>GAAASGSEFMPVSVEELDATVRAFYEGRGEQQKAAQAALNQFKEDPDAWLMVDEILSRATYEQTKFLALQVLDNVIMTRWKVLPREQCQGIRNFVVQYILQCSSSEESLRTHRTLLNKLNLVLVSVLKQEWPHNWPTFINEIVSACHSSLSVCENNMIILRLLSEEVFDYSADQMTSTKTRNLKSTMCAEFSMIFQLCQEILNSATQPSLIKATLETLLRFCNWIPLGYIFETPLIDTLRTRFLEVPEFRNVTLQCLTEIGGLQTGGPGQPHTYDEQLIKMFTEVLTTISNIIPLQMDLKATYPNSNSRDQEFIQNLALFLTSFFTMHLPLIENLPNRDFLTHGHFYLIRISQIDDREIFKICLDYWLKLVQELYEEMQSLPLNDMSSMGLGMMSGGGAPNPALLEHYPLRKHKYKEVLSNLRVVMIEKMVRPEEVLIVENDEGEIVREFVKDTDSVQLYKTIRECLVYLTHLDVVDMEQIMTEKLARQVDGSEWSWHNCNVLCWAIGSISMAMNEETEKRFLVTVIKDLLGLTEMKRGKDNKAVVASNIMYIVGQYPRFLKAHWKFLKTVVNKLFEFMHESHEGVQDMACDTFIKIAKQCRRHFVALQPSENEPFIEEIIRNIGKITCDLTPQQVHTFYEACGYMVSAQGNRNQQERLLAELMAIPNAAWDEIIKAATMNPGILHEPDTIKIIGNIMKTNVSACSSIGPYFFPQIGRLYNDMLQMYAATSQLISEAVARDGEIATKMPKVRGLRTIKKEILKLVETFVEKAEDLQAVRSQMIPGLLDSVLVDYNRNVPGARDAEVLKAM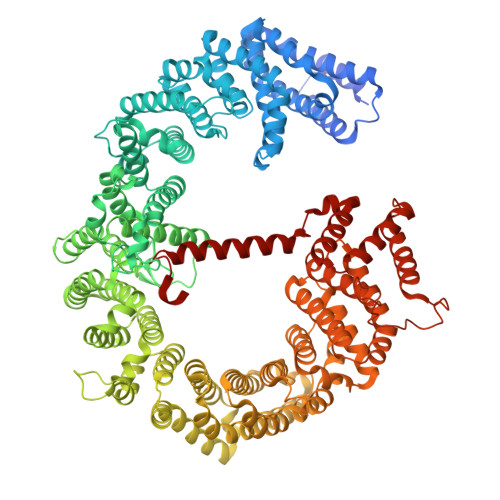TVIITRLQGLMEDQVPAIMENVFECTLDMINKDFAEYPEHRVEFFNLLRAINLYCFPALLKLDNRQFKFVIDSCMWASKHDNRDVETAGLNMCLELINNIAEKTDVQTCNAFFNQFFIRILQDVFFVLTDTDHKAGFKTQSMLLMRLFYFVHPADGSAPKIQGPIYQPDQAQPGTGNREFLANFVGTLLQNAFANLTPLQITTFVKDCFELNTQYDKFRVVLRDFLISLREFAGDNAELYQVEKEQQEREARAADLERRSKVGGLLKPSELEDEEL[2x]>[4x]TGDAAVALDTVTVVGE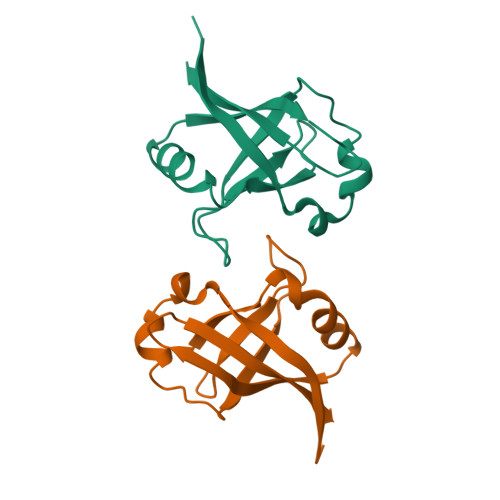RYVDDIVATLTTLRVGMAVLLQRESGNQYDDNAISVWTLQHAKLGYIARYQNQPYATLMDQGQRLYGIVTVLDQQKQHLELMLWRLEHHHHHH>SNAMKISDAVVSAHIDDEVVLLHLQTGTYFGLDAVGSRIWSLLEEGKRPEEIVDAICAEYSVDRPTVE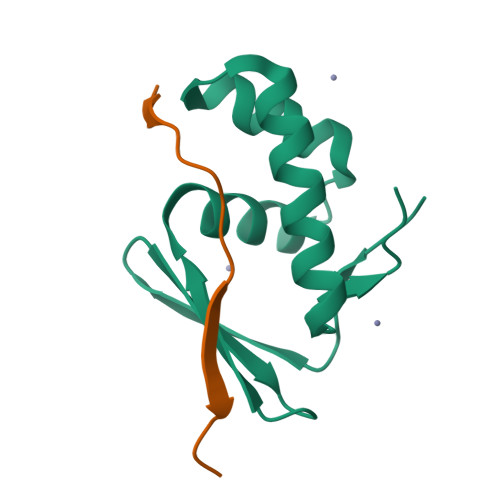RDLRDFLRALANKELLEGYADEA[2x];>MKEYRSPELKEYGRVEDRTAG[2x]> MDIELTKKDGTVIKLSEYGFIVNDIVIDSMQINTKYQDKENMNGRILMGSNYISRDIVVPCFCKVKNRSDIAYMRDMLYSLTTDIEPMYLREIRRKEELNYRFTQPTSDDYVKLDKNNFPDYEYSRHDQQIYVNGKQYKVIFNG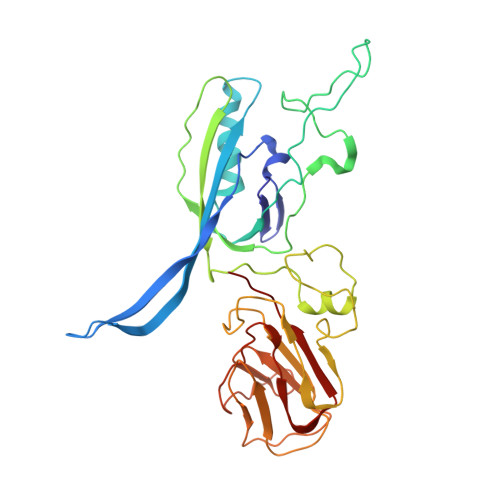VINPKQKGNKVSFELKFETTELPYGESIGTSLELEENKKVGLWSFDFNIDWHAGGDKRKYTFENLSKGTVYYHGSAPNDQFNMYKKITIILGEDTESFVWNLTHAEIMKIEGIKLKAGDRIVYDSFRVYKNGVEISTETNISQPKFKYGANKFEFNQTVQKVQFDLKFYYK Methylene‐tetrahydropterin reductases catalyze the reduction of a methylene to a methyl group bound to a reduced pterin as C1 carrier in various one‐carbon (C1) metabolisms. F420‐dependent methylene‐tetrahydromethanopterin (methylene‐H4MPT) reductase (Mer) and the flavin‐independent methylene‐tetrahydrofolate (methylene‐H4F) reductase (Mfr) use a ternary complex mechanism for the direct transfer of a hydride from F420H2 and NAD(P)H to the respective methylene group, whereas FAD‐dependent methylene‐H4F reductase (MTHFR) uses FAD as prosthetic group and a ping–pong mechanism to catalyze the reduction of methylene‐H4F. Mutational analysis of four functional amino acids, which are similarly positioned in the three reductase structures, indicated despite the insignificant sequence identity, a common catalytic mechanism with a 5‐iminium cation of methylene‐tetrahydropterin as intermediate protonated by a shared glutamate. Based on mutational and kinetic analysis, evidence has been provided that all three methylene‐tetrahydropterin reductases have the same fold, similar methylene‐tetrahydropterin binding positions, and the same basic catalytic mechanism; however, the binding modes of the C1 carriers and reductants significantly deviate.

Here, Mer from Methanocaldococcus jannaschii (jMer) was heterologously produced and the crystal structures of the enzyme with and without F420 were determined. Crystal structures for the apoenzyme of jMer and the binary jMer‐F420 complex were determined at a resolution of 1.8 and 1.9 Å, respectively. The active site of jMer is located in a cleft between the α/β‐barrel domain and a helix‐bundle subdomain composed of five helices. In the experimentally determined jMer‐F420 structure, F420 is associated with the α/β‐barrel domain with the isoalloxazine ring positioned at the bottom of the cleft in contact with the C‐terminal loops of most strands of the (αβ)8 barrel. The residual part of F420 pointing to the entrance of the cleft is sandwiched between the loops after β4 and β5 and reached the N‐terminal ends of the following helices. The cleft is sufficiently large to also accommodate methylene‐H4MPT with the pterin head adjacent to the isoalloxazine ring of F420. Gln178 is located close to the bottom of the cleft at the C‐terminal end of β6, which is presumably hydrogen‐bonded with the F420 isoalloxazine and the pterin ring. Glu6 at the C‐terminal end of β1 points towards the deaza‐isoalloxazine and pterin rings. The NPCP bond in jMer is located in the loop after β3, below the central pyridine ring of F420, between Gly61 and Val62.

>MKFGIEFVPNEPIQKLCYYVKLAEDNGFEYCWITDHYNNRNVYMALTAIAMNTNKIKLGPGVTNPYVRSPAITASAIATLDELSGGRAVLGIGPGDKATFDALGIEWVKPVTTLKESIEVIRKLLAGERVSYEGKVVKIAGAALAVKPIQKAVPVYMGAQGPKMLETAGMIADGVLINASNPKDFEAAIPLIKKGAEAAGRSMDEIDVAAYACMSVDKNADKAKQAAVPVVAFIAAGSPPVVLERHGIDMEKVEAIRNALKSGNFPEAFKNVDDTMLEAFSIYGTPEDVVEKCKKLAEMGVTQIVAGSPIGPNKETAIKLIGKKVIPALKE[2x]Type III secretion systems (T3SS) allow the transport of protein substrates directly across the double membrane of Gram-negative bacteria. Proteomic analyses have identified the major components of the sorting platform for the Salmonella typhimurium SPI-1 injectisome: the AAA+ ATPase InvC, its regulator OrgB and the proteins SpaO and OrgA4. Here we show that a novel, heterotypic interaction between SPOA domains serves as a scaffold for sorting platform assembly in both injectisome and flagellar T3SS. Our structures suggest a partial model for the subtype-specific assembly of the T3SS sorting platforms: the heterotypic interaction between SPOA domains within a given T3SS subtype functions as an adaptor for ATPase and its regulator through interaction with the APAR peptide.

The SpaO homologues FliM and FliN are predicted to contain one SPOA domain each, which we designate as SPOA1 and SPOA2, respectively. While complexes of FliM and FliN were stable, they were resistant to crystallization. Interestingly, FliM and FliN can be fused and still support flagellin secretion and some swarming motility. We crystallized the SPOA of FliM (residues 245–334) fused to FliN(5–137), and its structure was solved to 2.56 Å. Architecturally, the FliM(SPOA1)–FliN(SPOA2) interaction is similar to that of SpaO (2.28 Å r.m.s.d.), with the exception of additional helices present at the carboxy terminus of each SPOA, as observed in FliN homodimers from Thermotoga maritima. The similarity of these structures is consistent with the SPOA heterotypic interaction being generalizable across T3SS subtypes. In the context of our FliM–FliN structure, this suggests a model for FliM–FliN interaction similar to that of SpaO. FliM(SPOA1) would engage FliN(SPOA2) in a heterotypic SPOA–SPOA interaction, and additional homodimeric FliN would interact with FliM–FliN in an as of yet undetermined fashion (analogous to the SpaO SPOA2 homodimer interaction with full-length SpaO).

>GPVDNWRDNLVRQVQHSELELVANFADIPLRLSQILKLKPGDVLPIEKPDRIIAHVDGVPVLTSQYGTVNGQYALRVEHLINPILNSLNEEQPKNNPSDENTGALDDLWADALNEQKATTTKSAADAVFQQLGGGDVSGAMQDIDLIMDIPVKLTVELGRTRMTIKELLRLTQGSVVALDGLAGEPLDILINGYLIAQGEVVVVADKYGVRITDIITPSERMRRLSR[2x];> VFQQLG;> GALDDLWADELGRTRMTIKELLRLTQGSVVALDGLAGEPLDILINGYLIAQGEVVVVADKYGVRITDIITPSERMRRLSR2-[(1R,2S)-2-[5-[[(2S)-azetidin-2-yl]methoxy]pyridin-3-yl]cyclopropyl]ethanol 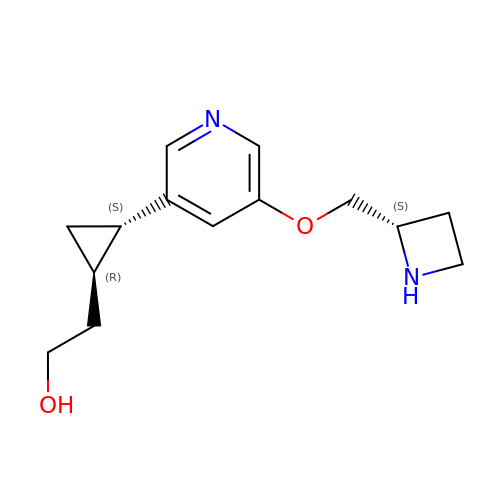| C14 H20 N2 O2 | FQIJPHXWIONJLF-JKOKRWQUSA-N>[16x]SPEEEQIIKELAKRKDIVDAIVDSIAPAIYGYKEVKKGIALALFGGVSRKLPDGTRLRGDI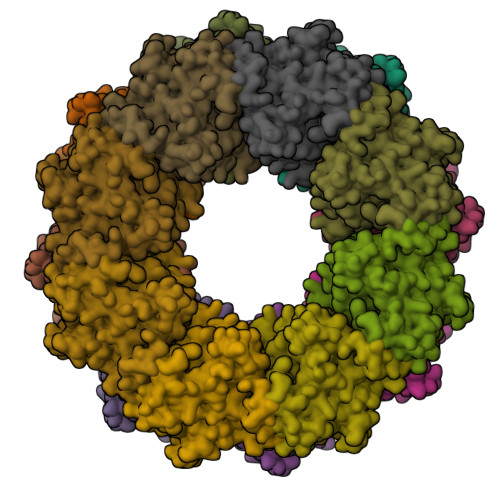HVLLVGDPGVAKSQILRYVANLAPRAIYTSXXXXXXXXXXXXXXXXXXXXXXXXXXXXXXXXXGGYALIDELDKMSDRDRSVIHEALEQQTISISKAGITATLNARTTVIAAANPKQGRFNRMKNPFEQIDLPPTLLSRFDLIFVLIDEPDDKIDSEVARHILRVRRGESEVVAPKIPHEILRKYIAYARKNIHPVISEEAMEEIEKYYVRMRKSVKKTKGEEEGIPPIPITARQLEALIRLSEAHARMRLSPIVTREDAREAIKLMEYTLKQIAMD>MTTPVLELLEQIQQGSEEQQKEALARLQELLEAGADPNMANSEGTTPVLLLLEIIQQGSEEQQKLALALLQELLEAGADPNMANSEGTTPVLLLLEIIQQGSEEQQKLAAALLKELLDAGADPNMANSEGTTPVLLLLEIIQQGSREQQALAMSLLLLLLLAGADPNMANSEGTTPKELLKEIQQQGSDEQRLLAEVLLQLLEAAGGSWGSHHHHHH[8x]

However, because of the intrinsic flexibility and irregularity of loop regions, organizing multiple structured loops at protein functional sites has been very difficult to achieve by de novo protein design. Here we describe a solution to this problem that designs tandem repeat proteins with structured loops (9–14 residues) buttressed by extensive hydrogen bonding interactions. Experimental characterization shows that the designs are monodisperse, highly soluble, folded and thermally stable. Crystal structures are in close agreement with the design models, with the loops structured and buttressed as designed.

The in silico validated designs span a diverse range of shapes with different repeat protein curvatures and loop geometries and adopt multiple loop buttressing strategies using loop–helix hydrogen bond networks and loop–loop bidentate hydrogen bonds. From a fundamental design perspective, the crystal structures presented here show that computational protein design has advanced to the point that proteins with multiple ordered long loops can now be designed. Key to this success was the design of dense networks of hydrogen bonding and nonpolar interactions within and between the loops and between the loops and the underlying secondary structural elements.>[4x]MANLNQKKYPAKDDFPNFEGHKSLLSKYLTADMYAKLRDVATPSGYTLDRAIQNGVDNPDFHLGLLAGDEETYTVFADLFDPVIEEYHNGF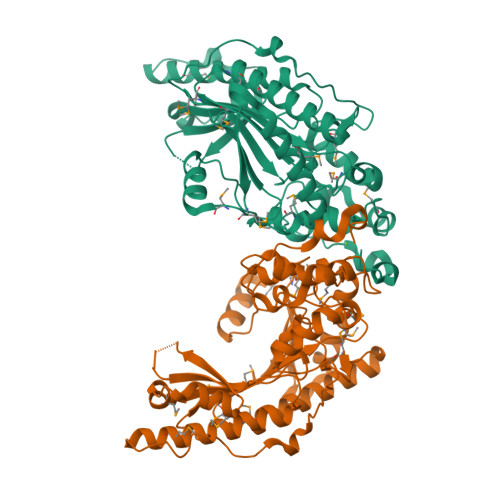KKTDNHKTDLDASKILDDVLDPAYVISSRVRTGRNIRGMALSPHVCRSERRAIEKMVSEALNSLAADLKGKYYSLMKMDEKTQQQLIDDHFLFDRPVSRHFTSGGMARDFPDGRGIWHNDKKNFLVWINEEDHTRIISMQMGGNMKEVFERFTRGLTEVEKHIKDKTGKEFMKNDHLGFVLTCPSNLGTGVRCSVHAKLPHMAKDKRFEEICTKMRLQKRGTSGEFTESVGGVYDISNLDRLGSSEVEQVNCVIKGVKVLIEMEKKLEKGESIDDLVPK SALT is a one such glycine rich Man-binding lectin known to be induced in rice under the effect of salinity, elevated ionic concentration, sucrose starvation, and water deprivation. Along with SalT transcript expression induced under different stress conditions, its expression is also found to be regulated by developmental and hormonal clues. These reports emphasize on the key role of SALT protein in regulation of multiple processes including plant growth, development and stress responses. The present work delves with the detailed structural characterization of SALT protein in complex with mannose both in solution as well in crystalline state using SAXS data analysis and X-ray crystallography, respectively. Overall, our studies unequivocally prove that SALT exists as a tightly bound dimer.

From crystals grown at 18 °C, we could acquire diffraction data up to 1.66 Å. The crystals were monoclinic with P1211 space group with two molecules of SALT in each asymmetric unit. The structure of SALT protein is predominantly composed of β-sheets (66.2%) and remaining is random coil or unstructured loops interconnecting them. There are 3 β-sheets, each composed of 4 β-strands. Interestingly, two molecules of mannose are also present in the asymmetric unit, each bound to a protein chain. Each mannose is bound to the protein through 8 H-bonds involving protein residues Gly14, Gly133, Thr134, Leu135, and Asp137. In our structure of SALT protein, both the loops are closer to the main body of the protein and have significantly lower B-factor indicating a more stable conformation. This might be the result of the bound mannose or the two mutations i.e. G62S and H74Q, which are located in vicinity of the loops. Importantly, the computed SAXS profile of our crystal structure of SALT protein is in excellent agreement with the experimental SAXS profile with a χ2 value of 1.5 indicating the dimer structure seen in our crystal structure is present in solution as well.

>MTLVKIGLWGGNGGSAQDISVPPKKLLGVTIYSSDAIRSIAFNYIGVDGQEYAIGPWGGGEGTSTEIKLGSSEHIKEISGTHGPVYDLADIVTYLKIVTSANNTYEAGVPNGKEFSIPLQDSGHVVGFFGRSGTLIDAIGIYVHP[2x]FMDV is the causative agent of foot-and-mouth disease, a highly infectious disease of cloven-hooved animals. Final processing of P3 is thought to occur through both major and minor pathways via a differential set of intermediary precursors to ultimately produce the 3A transmembrane protein, three nonidentical tandem copies of the primer polypeptide 3B (3B1–3), the major viral protease 3C, and the RNA-dependent RNA polymerase (RdRp) 3D (also known as 3Dpol). The crystal structures of 3D alone and in complex, e.g., with RNA and the primer peptide 3B (also known as VPg) have shed light on the mechanism of RNA polymerization. In summary, we have identified novel cis and trans functions of the FMDV 3D RNA-dependent RNA polymerase that are essential for viral RNA replication.

From this we concluded that disruption of residues G216 and C217 was responsible for the replication-defective phenotype in the dsRNA exit site. In contrast, neither of the dsRNA exit site point mutations (3D-GC216/7AA or 3D-GCNP216-9AAAA) was recovered, with no significant increase in ptGFP expression when cotransfected with helper construct compared to yeast tRNA control. The X-ray structure of the 3D-GC216/7AA polymerase, in complex with the RNA template/primer 5′-GCAUGGGCCC, was solved at 2.8-Å resolution. The initial difference maps allowed unequivocal tracing of the substituted (GC216/7AA) and surrounding (from V215 to D220) residues that were omitted from the initial model to eliminate model bias. These maps also indicated the presence of the duplex portion of the template-primer in the central cavity of the enzyme and the AU nucleotides, belonging to the template 5′ overhang region, bound to the template channel. Structural comparisons showed that the 3D-GC216/7AA mutant polymerase is almost identical to the wild-type 3D. Structural comparisons also showed a subtle movement of the loop containing the mutated residues GC216/7AA, which was displaced by ∼0.74 Å toward the RNA primer. However, this small displacement does not alter the 3D-RNA interactions at the dsRNA exit site. The main differences lie in the template entry channel, in particular in the M16-R17 segment, located distal from the mutated region. In contrast, in the GC216/7AA structure, the main and side chains of residues M16 and R17 appeared reoriented, with the R17 side chain pointing to the polymerase interior, interacting with residues N41 and Y285.

> GLIVDTRDVEERVHVMRKTKLAPTVAHGVFNPEFGPAALSNKDPRLNEGVVLDEVIFSKHKGDTKMSAEDKALFRRCAADYASRLHSVLGTANAPLSIYEAIKGVDGLDAMEPDTAPGLPWALQGKRRGALIDFENGTVGPEVEAALKLMEKREYKFACQTFLKDEIRPMEKVRAGKTRIVDVLPVEHILYTRMMIGRFCAQMHSNNGPQIGSAVAANPDVDWQRFGTHFAQYRNVWDVDYSAFDANHCSDAMNIMFEEVFRTEFGFHPNAEWILKTLVNTEHAYENKRITVEGGMPSGCSATSIINTILNNIYVLYALRRHYEGVELDTYTMISYGDDIVVASDYDLDFEALKPHFKSLGQTITPADKSDKGFVLGHSITDVTFLKRHFHMDYGTGFYKPVMASKTLEAILSFARRGTIQEKLISVAGLAVHSGPDEYRRLFEPFQGLFEIPSYRSLYLRWVNAVCGDAAAALEHHHHHH>[2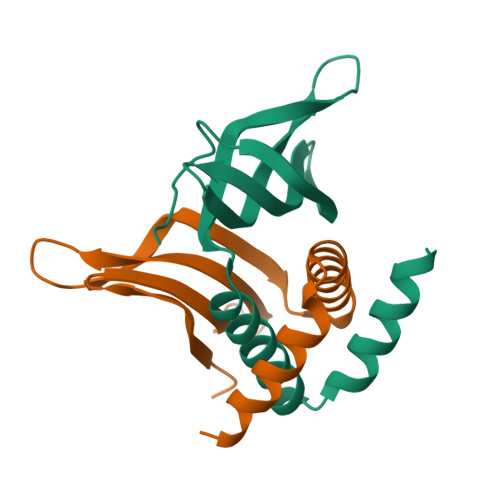x]MSEQVNQNYEGHVDDQSIILWEKEGEQVRLTVSEFRGNLYMGIRYWLLDINDEWFPTKSGFSFPYTLETTSQLFYAFTQILSESEVLHEVQKRAEELKAKNA>[3x]KVEIIRGDHPEVYDDSAENEVPTAASIQRKAILETLTNLMLESQTPGTRQIREEESTIPIFAESTTQKTISVSDLPNNCLNASSLKCEIKGISTYNVYYQVENNGVIYSCVSDSAEGLEKCDNSLNLPKRFSKVPVIPITKLDNKRHFSVGTKFFISESLTQDNYPITY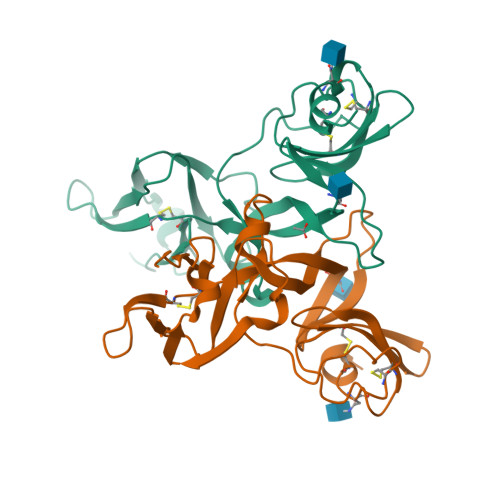NSYPTNGTVSLQTVKLSGDCKITKSNFANPYTVSITSPEKIMGYLIKKPGENVEHKVISFSGSASITFTEEMLDGEHNLLCGDKSAKIPKTNKRVRDCIIKYSKSIYKQTACINFSWIR>TGGGTTGGGTTGGGTTGGGT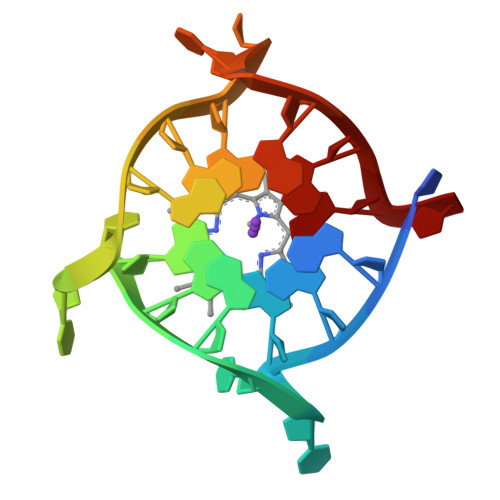[2x]The viral genome is encapsidated in a sheath of oligomerized copies of the nucleoprotein N, forming a ribonucleoprotein complex termed nucleocapsid. The nucleocapsid is the template for transcription and replication by L, which is also dependent on the obligate polymerase cofactor, the phosphoprotein P, together forming the active L/P holoenzyme. In oligomerized and RNA-bound N (N-RNA) the nucleic acid is threaded along an extended groove in between the NTDs and CTDs of laterally connected N protomers. An important function of the C-terminal domain of P in nsNSVs is to bind to assembled N-RNA, forming an N-RNA/P complex.

We incubated N-RNA preparations with a ~ 100-fold molar excess of synthetic peptide covering the 9 last residues of PCT (N-EDDIYQLIM-C). Cryo-EM analysis of the N-RNA/P complex revealed the presence of the same classes of assemblies as was the case with the apo sample. We carried out 3D reconstruction of 10-mers, 11-mers, and spiral particles of the N-RNA with PCT. In the reconstructions, additional density was visible at the periphery of the NTD of N. To facilitate easier model building and to obtain improved maps, we carried out symmetry expansion and local refinement of a dimer of N-RNA/P as before with N-RNA. P binds into a groove at the periphery of the NTD of N, between a helix and an extended loop of a beta-hairpin of N (here denoted as NβHL). We observed that the density of NβHL becomes more ordered upon P binding, indicative of a folding-upon-binding event. Lastly, viewed in the context of an N-RNA assembly, the PCT binding site is located such that P attaches to a region of the nucleocapsid that protrudes at a far radius from the helical axis.

> MSLQGIHLSDLSYKHAILKESQYTIKRDVGTTTAVTPSSLQQEITLLCGEILYAKHADYKYAAEIGIQYISTALGSERVQQILRNSGSEVQVVLTRTYSLGKIKNNKGEDLQMLDIHGVEKSWVEEIDKEARKTMATLLKESSGNIPQNQRPSAPDTPIILLCVGALIFTKLASTIEVGLETTVRRANRVLSDALKRYPRMDIPKIARSFYDLFEQKVYHRSLFIEYGKALGSSSTGSKAESLFVNIFMQAYGAGQTMLRWGVIARSSNNIMLGHVSVQAELKQVTEVYDLVREMGPESGLLHLRQSPKAGLLSLANCPNFASVVLGNASGLGIIGMYRGRVPNTELFSAAESYAKSLKESNKINFSSLGLTDEEKEAAEHFLNVSDDSQNDYE;> DIYQLIM>[2x]MTATASGAQTAAPERLTDDGWLIRRTSVDTVRPFDDPSAQWMLDRAQARLPLYLLHVADHAEATPPGLREALHAQDAAPCDGLLFSQYGLPELRRRLDAWLAADEEWDTAAEPLVSVAWSGTGAAIFDLLRMLKDGRPGPSAVLLPRPGWGYDMSVRDTGHVPVSYEVPPESPHGPDP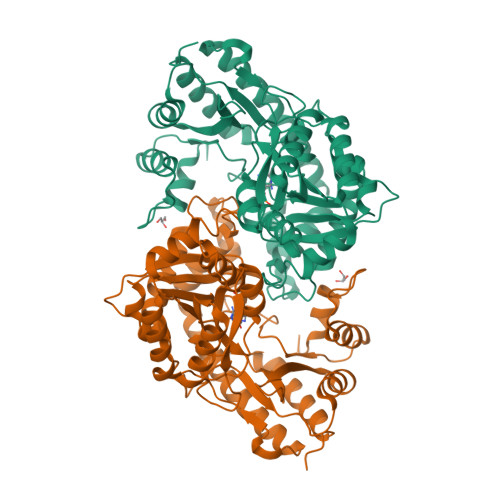AHLEEAWQRCRSEGLDVACILINPQHNPWGGNWTPEFLAAVAALAERERVPVLVDNAFYGLTAEDVRPTSAVRLLGHLVGQELLVSVRSLSKQFACSGWALGAVAGSPGLVSAYSGRWRCLREPTAGFRAQAAMAAWLGGAEPERFTRRRRSEATRHARLLRTTLRAAGLPDDAVLHHGGAPFTLLRPPGGSTVEEVREQTVVRHGVLLGLERDARERPWFKVWLGRDSSVFEPAARALGDAAAEWRYRLEHHHHHHHH>GAMAMTTDEGAKNNEESPTATVAEQGEDITSKKDRGVLKIVKRVGNGEETPMIGDKVYVHYKGKLSNGKKFDSSHDRNEPFVFSLGKGQVIKAWDIGVATMKKGEICHLLCKPEYAYGSAGSLPKIPSNATLFFEIELLDFKGEDLFEDGGIIRRTKRKGEGYSNPNEGATVEIHLEGRCGGRMFDCRDVAFTVGEGEDHDIPIGIDKALEKMQREEQCILYLGPRYGFGEAGKPKFGI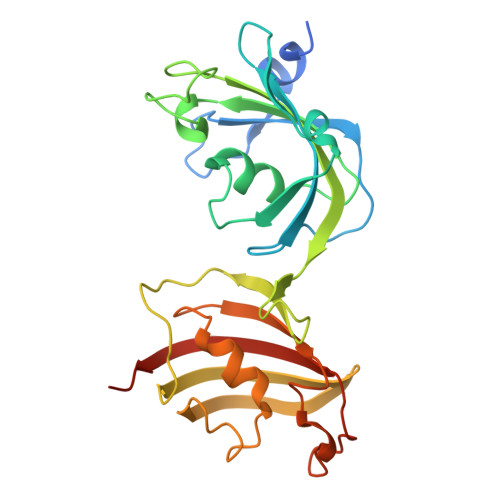EPNAELIYEVTLKSFEKAKESWEMD[2x]>[2x]HMINGSIVALITPLNSDGTVDYTSLEKLVEYHITEGTDAIVAVGTTGESATLPISEHIAVVGQTVKFASGRIPVIGGNGANATAEAIEL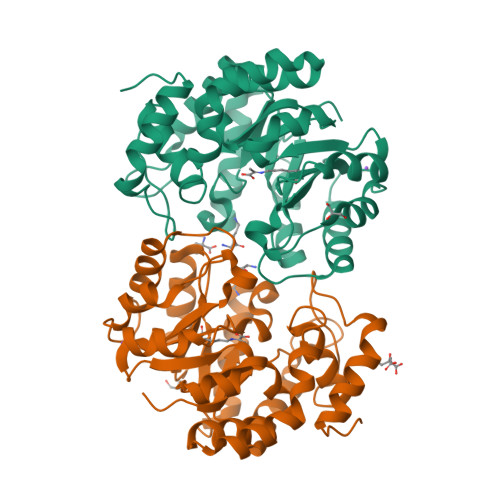TKAQNKLGVAAMLGVTPYYNKPSPKGLIAHYTAVAASTDIPQILYNVPGRTAVDMLPETIAQLVEVPNIIGVKDATGDVARVKQLRDLCGNDFLLYSGDDATAREFLTLGGDGVISVANNIVPKLFKLMCDAALAGDTQAAMAAEDQIKGLFSALFCEANPIPVKWAAHKMGLISQGDIRLPLTELSTEFHGLLLDAMKNARIEVK> MACQVDNPPKTYPNDKTAEYEKYANYMNYLYYYQNNELKKIDSSYFKDKYLGLFFGASWCKYCVTFIDSLNIFKKNFPNVEIIYIPFDRTYQEYQSFLKNTNFYALPFDNYLYICKKYQIKNLPSFMLITPNNNI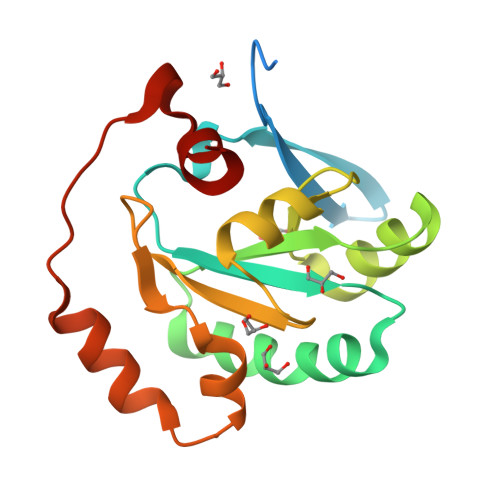LVKDAAQLIKTDEYINNLKSLIKNYIIHPKTFQFNNRFFDLFRN> MMYKEPFGVKVDFETGIIEG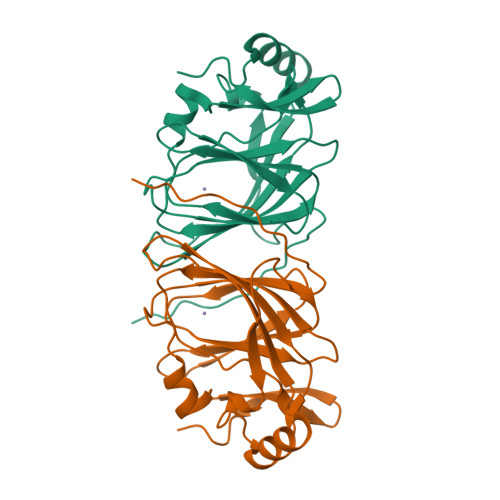AKKSVRRLSDMEGYFVDERAWKELVEKEDPVVYEVYAVEQEEKEGDLNFATTVLYPGKVGKEFFFTKGHFHAKLDRAEVYVALKGKGGMLLQTPEGDAKWISMEPGTVVYVPPYWAHRTVNIGDEPFIFLAIYPADAGHDYGTIAEKGFSKIVIEENGEVKVVDNPRWKK> MGSSHHHHHHSQDPENLYFQSMIPQFVIPLTNCLGQSYHFSSQPIPKGEHKKFDSEQSAKAFLDDFVPLRSSRVEELYHLLGQFPPNVPDEELTPELYAPVFAKALVNGSLYVASFPKTKKNATISSEPTPVPKQVKAKSKQNKAHTSSKTQAKNSASAKPLQTGSECHEKAGDPVSLVTGEEILTLNDVELPNGFVWSRTYRSSKASRNQGLGYGWRHAFQFELKEVTDEKHNVTSWEFISDSADEIEFEPVEHGSTSYQVYVGASCHFLNPNIRIVTLSSGDQYRFELVEDIWLLKQVRNGIFSTFQLRYSRNHRLIEVAHNKRPVLECQYDKQGRLVELLNAKTEQVLTTYIYDEQDDLVGATNDLGLTERYEYQDQHLIAKRVRPTGFTHYFEWSGEGSSAKCIRNFGDSGIYDYRFHYEGAKSSYSDSLDNEWTFIHDEQGHLLEKSSPTGRTWQWHYDHLGRKEKAVFPDNSTTQYQYNQQGQLISKLHSSGAQIQYGYDSLGKLVKTVSPDGDLEKAYYNSLGQRVWDIDALGCVTEYEYDKHGQVVKRESEDGKKSRWWWDKQQRLVAHEVDGTLLRYSYGATDLVNGIAYPDGCVAQISYDDYGRRTSIRYFNDEDKVGYSEEYAYDEFSRVAQIQTPEGVTSYQWGALAQQEAVIFPDGSHISYEYDQQRNLTKLVRSDGLAFEFWYDSEGLLSGTVGFDGLHSQFKYDSMGRIIRKDVADRTVLYSYDDAGFLQHIKAGNGKNIVENHFNYTLGGRLTLASNRHQTLQYQYSSFGHLTKRIQGQFEIGEEFNRVGQRVSQTLPDKTSFNFSYDTNGRLSEIRFSDDSLPKIEFQYDVMGRLSVTETESFRESKLYDGVGRLVEQQWSGREKKYIYNAQNRISSILDNTAGATHYQYDTLGYVTKVSEAGSTSTFESDSFGNPALADSKVMSDRIEAYAGVRYKYDQQGNQVKREGDGTVQKRVFDALSQLVEVHGDSSISHYEYDALGRRTKKITQNGITEFLWEGERLLGERTADGFRWYLYQPETYIPLAVLENGSIYLYECDQVGKPERLKDSAGNIVWSASYDVHGFASIDVEEVRNPLRFQGQYFDQETNLHYNLARYYDPKLGRFIQQDPISIAGGINHYQYAVNPIQWIDPTGF;> LCEEGLKRLQQMLAEYQAQSDVPQEVCDQILEAAKESSVGEDGVRSQVKIRKPNGKNNIRYEYDLDHIDCKKNEITFYRHINYSDGSKRKIQYTVGIEGFVDIYDFVNVQKCD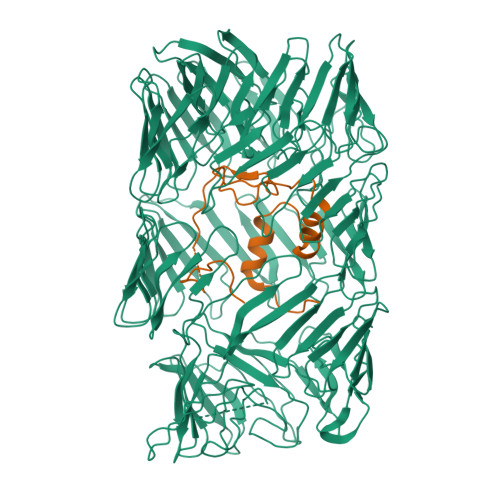AQVYDTKTSKTVGGRKIINSEFAGKTVTTKGGDVRFDSDGFPDFTPYSKKTVRVIGLTGDMANDVPLAMARAKITKYDKSKYVWHHHQDGKTMMLIPKSVHSVRNGGVAATGGRSVIQHNLLNPNNKLNYSSPEELV> MKKYTCTVCGYIYNPEDGDPDNGVNPGTDF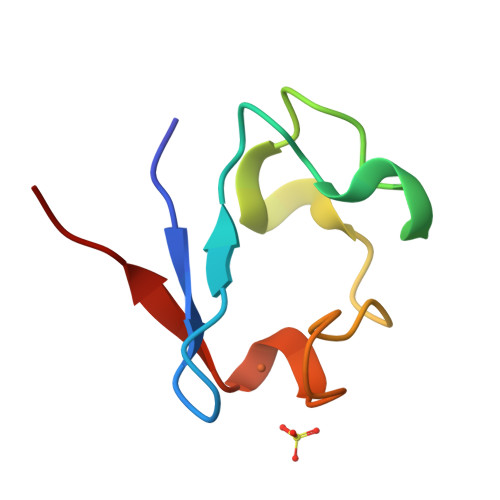KDIPDDWVCPACGVGKDQFEEVEE> G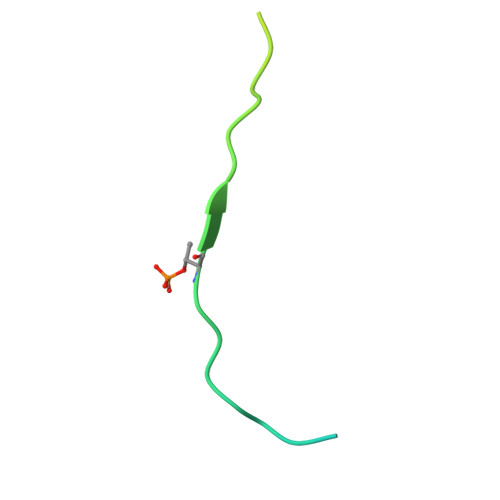VLPKAPKLQASQATLARQDTIDEGGEVDSSPPSRDSRVVIEGAAVSSATVGPS>[4x]GMAEPKFTSFTTADFINDVDMELFIDAVEKTAPVWVKEMKSRGLLKFSMNR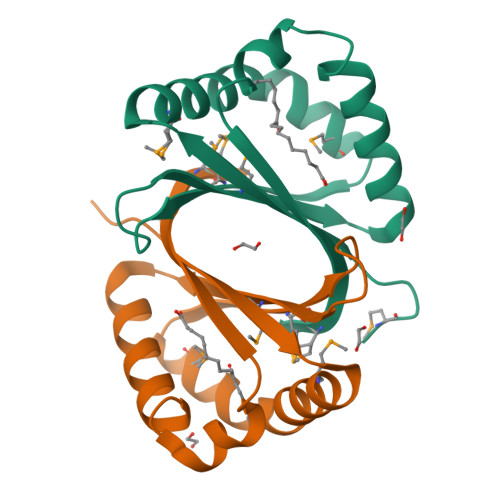VWNKGEVFRVVMTYEYKDRASFEANIAYLEDTFGKNPVFLQLVTTAKFTTSRCLVVMEV The RsiG–WhiG cognate pair is the only known example of a σ–anti-σ complex that is targeted by c-di-GMP. Here we show that the same σ–(c-di-GMP)–anti-σ switch has been co-opted during evolution to regulate distinct biological functions in unicellular and filamentous bacteria, controlling type IV pilus production in the genus Rubrobacter and the differentiation of reproductive hyphae into spores in Streptomyces. Moreover, we show that the anti-σ likely originated as a homodimer and evolved to become a monomer through an intragenic duplication event. Structural analyses revealed that these single-motif RsiGs form an antiparallel coiled-coil through homodimerization, enabling them to bind c-di-GMP in the same manner as the monomeric twin-motif RsiGs.

Two well-diffracting crystal forms of the RsiGRr protein were obtained. Crystal form 1 was solved by selenomethionine single-wavelength anomalous diffraction (SAD) and refined to Rwork/Rfree values of 17.3%/20.2% to 1.86-Å resolution. The structure contains six molecules of RsiGRr in the crystallographic asymmetric unit (ASU), which form three essentially identical antiparallel dimers (root mean square deviations of 0.6 Å when comparing Cα atoms of the coiled-coils). Indeed, the structure shows that the single-motif RsiG from R. radiotolerans is homodimeric, with helical residues 45 to 83 forming a tight antiparallel homodimeric coiled-coil with overall structural similarity to the monomeric twin-motif RsiG from S. venezuelae. The formation of the homodimeric RsiGRr coiled-coil buries an extensive 1,904 Å2 of protein surface from solvent. This corresponds to a predicted ΔG solvation free-energy gain upon interface formation of −35 kcal/mol, supporting that the homodimer is the physiological relevant form. The same RsiGRr crystal forms were obtained in the presence of c-di-GMP under identical crystallization conditions, but no nucleotide was visible in the structures. This appears to be due to the presence of Mg2+ ions, which were required for crystallization for both crystal forms. The Mg2+ ions in both apo structures are coordinated by D74, located at the C terminus of the E(X)3S(X)2R(X)3Q(X)3D motif. The tightly coordinated Mg2+ in the RsiGRr structure sterically disallows c-di-GMP binding.

>[6x]GSHMRESAEEVWGGTEDLTSLSVEELKGLMARFDEEEKRISYRRRVMQGRIDVIRAEIVRRGGAVLSPEELARVLMGDVGDESE Calsequestrin (Casq) is considered to be the major Ca2+-storage/buffer protein within the sarcoplasmic reticulum (SR) of both cardiac and skeletal muscle, where it resides as either its cardiac (Casq2) or skeletal (Casq1) isoform. Casq binds Ca2+ with a capacity roughly equivalent to a half of its total negative charge and an overall dissociation constant of ~1 mM. When studied in solution, Casq polymerizes as free Ca2+ concentrations increase and depolymerizes as Ca2+ concentrations decrease. We also showed that both glycosylation and phosphorylation alter the physical characteristics of Casq substantially, including its oligomerization and Ca2+-binding capacity.

To investigate any structural significance/role of glycans or structural change due to the presence of glycans, the crystal structures for both native and recombinant bovine Casq1, which correspond to the glycosylated and nonglycosylated form, respectively, were determined under the same condition. Calsequestrin crystallized in two forms: the low-Ca2+ forms of native and recombinant bovine Casq1 crystallized in the absence of added Ca2+ in the crystallization buffer; the high-Ca2+ forms crystallized in the presence of 2.5 mM Ca2+ (17× molar excess of Ca2+ added to solution). Low-Ca2+ native bovine Casq1 crystallized in the P1 space group and contained four molecules in the unit cell; the resolution of its diffraction data was 2.74 Å, whereas low-Ca2+ recombinant bovine Casq1 crystallized in the C2221 space group and contained one molecule in the asymmetric unit, with a resolution of 1.88 Å. The lattice packing for both low-Ca2+ native and recombinant established a typical weakly-interacting linear polymer with D2 symmetry, a pattern also found in previous Casq structures. Each monomer in the low-Ca2+ structures of both native and recombinant Casq1 contained five Ca2+ ions, while the three monomers in the high-Ca2+ asymmetric units contained a total of 38 Ca2+ ions. In the case of low-Ca2+ native Casq1, the glycosyl groups on the four molecules in the crystallographic asymmetric unit modeled reliably into the corresponding electron density map as GlcNAc2 for two monomers, GlcNAc2Man1 for another monomer and GlcNAc2Man2 for the remaining monomer. Superposition of low-Ca2+ recombinant Casq1 onto the four low-Ca2+ native monomers in the P1 unit cell had an average r.m.s.d of 0.40 Å.

>EEGLDFPEYDGVDRVVNVNAKNYKNVFKKYEVLALLYHEPPEDDKASQRQFEMDELILELAAQVLEDKGVGFGMVDSEKDAAVAKKLGLTEEDSVYVFKGDEVIEYDGEFSADTLVEFLLDVLEDPVELIEGERELQAFENIEDDNKLIGYFKNKDSEHYKAYEDAAEEFHPYIPFFATFDSKVAKKLTLKLNEIDFYEAFMEEPVTIPDKPNSEEEIVSFVEAHKRSTLRKLKPESMYETWEDDLDGIHIVAFAEETDPDGYEFLETLKAVAQDNTDNPDLSIIWIDPDDFPLLVPYWEKTFNIDLSAPQIGVVNVTDADSVWMEMDDEEDLPSAEELEDWLEDVLEGEINTEDDDEEDD[4x]> DDKLPRYIAGVLARLQEVWLGRQIA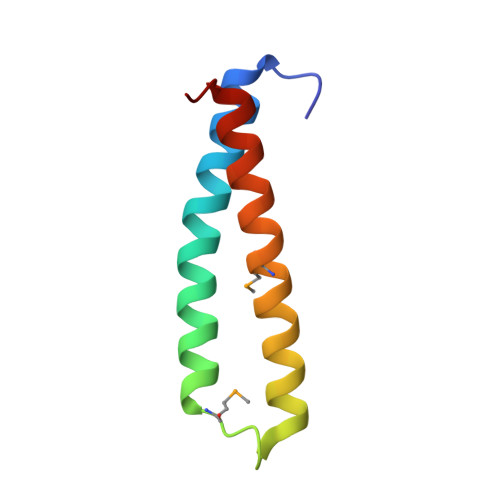EVKSKLQRMSPIEQGDEYHALFGDLVAMEAYRRSLLEQASGDDLHH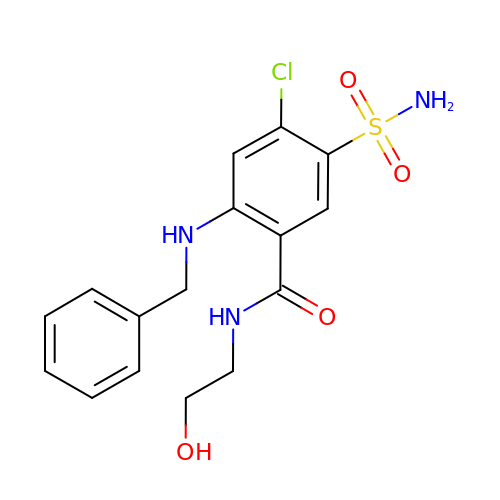4-chloranyl-~{N}-(2-hydroxyethyl)-2-[(phenylmethyl)amino]-5-sulfamoyl-benzamide | C16 H18 Cl N3 O4 S | JHJVKSXZTYMHHX-UHFFFAOYSA-N>[2x]GSQQRKVLTLEKGDNQTFGFEIQTYGLHHREEQRVEMVTFVARV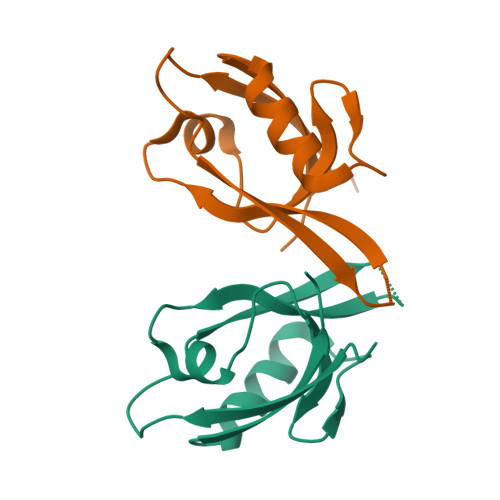HESSPAQLAGLTPGDTIASVNGLNVEGIRHREIVDIIKASGNVLRLETLYGT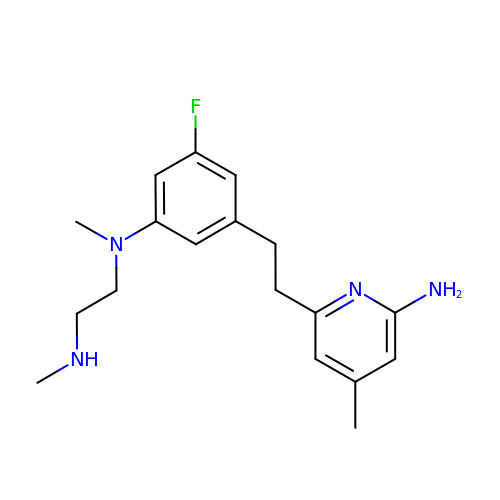N1-(3-(2-(6-AMINO-4-METHYLPYRIDIN-2-YL)ETHYL)-5-FLUOROPHENYL)-N1,N2-DIMETHYLETHANE-1,2-DIAMINE | C18 H25 F N4 | ZVNKMLXKHZSKMN-UHFFFAOYSA-N> MDVVSLDKPFMYFEEIDNELDYEPESANEVAKKLPYQGQLKLLLGELFFLSKLQRHGILDGATVVYIGSAPGTHIRYLRDHFYNLGVIIKWMLIDGRHHDPILNGLRDVTLVTRFVDEEYLRSIKKQLHPSKIILISDVASAAGGNEPSTADLLSNYALQNVMISILNPVASSLKWRCPFPDQWIKDFYIPHGNKMLQPFAPSYSAEMRLLSIYTGENMRLTRVTKSDAVNYEKKMYYLNKIVRNKVVVNFDYPNQEYDYFHMYFMLRTVYCNKTFPTTKAKVLFLQQSIFRFLNIP;> PNITLKIIETYLGRVPSVNEYHMLKSQARNIQKITVFNKDIFVSLVKKNKKRFFSDVNTSASEIKDRILSYFSKQTQTYNIGKLFTIIELQSVLVTTYTDILGVLTIKAPNVISSKISYNVTSMEELARDMLNS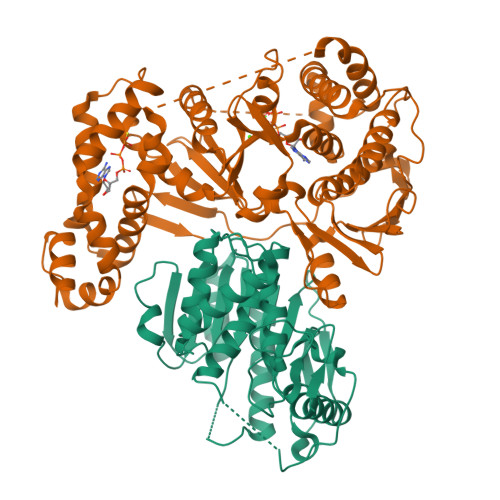MNVAVIDKAKVMGRHNVSSLVKNVNKLMEEYLRRHNKSCICYGSYSLYLINPNIRYGDIDILQTNSRTFLIDLAFLIKFITGNNIILSKIPYLRNYMVIKDENDNHIIDSFNIRQDTMNVVPKIFIDNIYIVDPTFQLLNMIKMFSQIDRLEDLSKDPEKFNARMATMLEYVRYTHGIVFDGKRNNMPMKCIIDENNRIVTVTTKDYFSFKKCLVYLDENVLSSDILDLNADTSCDFESVTNSVYLIHDNIMYTYFSNTILLSDKGKVHEISARGLCAHILLYQMLTSGEYKQCLSDLLNSMMNRDKIPIYSHTERDKKPGRHGFINIEKDIIVF> AIYEKAKEVSSALS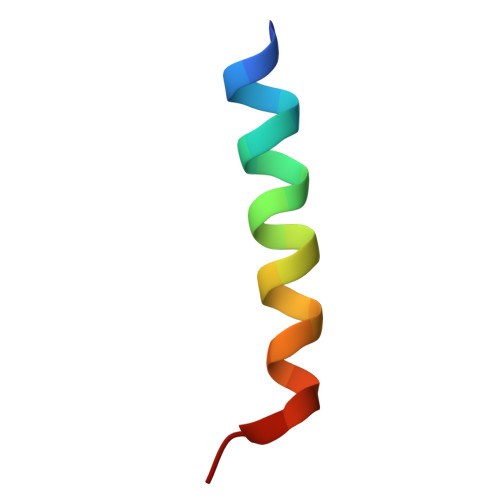KVLSKIDDT Many of the HK and MCP signal transduction proteins span the cytoplasmic membrane and detect extracytoplasmic signals/stimuli via “sensor” domains that face the periplasm. Binding of a small molecule or other stimulus to these domains initiates a response in the cytoplasmic domains, which in turn triggers the downstream regulatory processes. We have undertaken a study of the periplasmic sensor domains from A. dehalogenans 2CP-C with an eventual goal of delineating the functions of some of the signal transduction proteins (The term “signal transduction proteins” hereafter is used to refer to transmembrane sensor histidine kinases [HK] and methyl-accepting chemotaxis [MCP] proteins only) from this organism. Although sensor domains have been studied for many years, there are still many unknowns about the actual ligands that stimulate a given response and the mechanism of signal transduction. It is now apparent that both HK and MCP proteins interchangeably use the PAS-like (including tandem PAS-like) and helical bundle sensor domain tertiary folds.

Periplasmic sensor domain (residues 38–190) of chemotaxis protein, Adeh_3718 was isolated, purified, and crystallized as described in the methods section. Adeh_3718 crystallized in space group P3121 and diffracted X-rays to 2 Å resolution. The crystals consist of one protein molecule per asymmetric unit and there is no indication of oligomeric interactions in the crystal as determined by the PISA server. The PAS-like domain of Adeh_3718 consists of two N-terminal helices α1 (residues 41–68), α2 (residues 72–87), followed by two small β-strands β1 (residues 96–100) and β2 (103–106), helix α3 (residues 110–114), helix α4 (residues 128–141), β3 (residues 142–151), β4 (residues 156–167), and β5 (residues 171–180). The structure of Adeh_3718 sensor has revealed a fully occupied acetate ion moiety bound to the protein in this binding site. The acetate ion is bound stacked between two tryptophan rings of Trp96 and Trp149. Salt bridges are observed between the carboxylate group of acetate ion and side chains of Lys160 and His107. Two additional hydrogen bonds are made with the side chains of Tyr94 and Tyr147. The methyl group of the acetate is facing a hydrophobic pocket lined with the side chains of Leu129, Phe130, and Phe133. Although PAS-like domains can bind ligands nonspecifically and acetate binding by Adeh_3718 sensor may just be a crystallization artifact, one cannot rule out the possibility that Adeh_3718, which is a chemotaxis protein, could be involved in sensing environmental acetate by A. dehalogenans.

> ARMLAERQAKVRALVEAAHGLVEHQGARAARGEISADEARRAALEALRALRYDGSEYFWVNDLEPRMVMHPTNPQLDGQDLSGYRDPNGKLLFQEFVRTVRARGSGFVDYLWPKPGSTVPVPKISFVTQYQPWGWVVGSGLYVDDLDAAVRQE> SNAQDANHSSNNKDTEKSDKKYHRII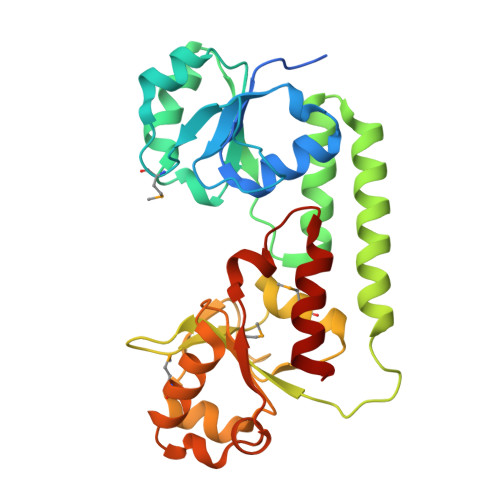SLIPSNTEILYRLGIGEDIVGVSTVDDYPKDVKKGKKQFDAMNLNKEELIKAKPDLILAHESQKNSAGKVLKSLKDKGVKVVYVKDAQSIDETYDTFKSIGQLTDREKQAKELVDETKHNVDKIINSVPKHHKKQEVFMEVSSKPDIYTAGKDTFFNDMLEKLDAKNSFDDVKGWKSVSKESIIKRNPDILISTEGKSKSDYIEMIKKRGGFDKINAVKNTRIETVDGDEVSRPGPRIDEGLKDLRDDIYKK> MSNNRDLPKNPLIRDGVSQRQRQVSALSPASIGVDERDLADFLVLVYRLSAKVMYYRAENQPWSPSDADGNWQNFFEGNTPIQIALISKVSPQVVKDIYSQKLAAFLAERTVTSLSEVLSIWKTEILTKIQQWYLGIEAYTPLKSVIKGLVKTNLTEPLMRMQSFELGCGNVDEEFYRGFSGVFGLTIDAPLRSDRTPLMGTVKDARTELDTVFQVLLQTYRQIIQQAPNYLKASLSDRQDHQPFLSLYFAFLEVLQPARDDLNRLTQRHLDFFYRQVLLLPDRPAQADQVHLLFELAKSQREYKLTAGTSFKAGKDATGVDLFYQLDAETVIHKAQIASLKGLFLDSQERKTAAVPQNLTGLYASPVANSVDG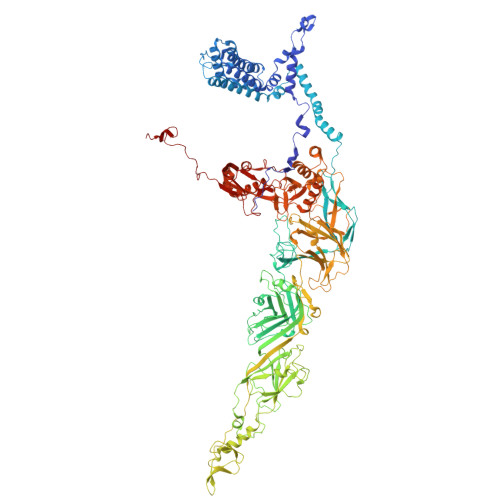KGGAFPQEQIVKTWLPFGNEQRDHARLGVAIASDVLLLQEGRRVVEFKLSLGGFFPRLPDNQLHQAFVVYLSGEKAWIPAPILPVGQLATNGQEQTRWDGSNLYLVVELAADVAPILPYRPDAPIPYDPKELNLPLQLERPIPVARLELNHQLLVNERSPYHYFRDAQILDITVQTRVDEVRNLVVQNDVSVLNPARPFEPFGFQPQDKANLYIGSQEVLQKRLIALTISLELATPKPNNWIEFYAGYDIPANFQPGKVKIQGLRQKTWYPTTANVTANLLDTPEISLTSKLANLKLDSFDQSAPVEMFTPQTKTGFLRLQLSGNFLHEQYPRVLAKQVLAAATNQTVVVSSNQKRQAVIGAYYRRPDKSIFAATTYYVNLDDEPIIPNEPYLPVVRSLSLKYTAQAGMSDCILFHLHPFGGFAKVNLAVNPPLLPYFNQEGELFIGLQNLDPPTALPLLFQVAEETADISLRRQEEYKLQWYYLKDNAWESLGDRIVNDASNGLVTSGIINLGIPADISRNQTTILDPNFHWLKVTIPARSRTVCEIIGVHTQAARVTFKDAGNDPNHLGSPLAGGTISKLAVPQPEVKKIAQPYTSFGGRVKEQPENFYIRISERLRHKGRAVAIFDYERLVLEKFPQIYKVRCINHGQFDDAQEQLYELAPGSVTLAVIPDLSQRSTTNDLEPKVNINLLQEIEKYLASVSSPWAMIKVVNPQYERIQVDFQVKLKAPYSSNFGYYRRELQQAIVGFLTPWTVDSGADINFGGKVYRSSILKFVEEQYYVDYVVNFKMNLNNQQDIREAIAITPRSVITSVSPKTSNQDHMIEEFIEQAIVFNNQKLESGVLGYESLNDLELGE Unlike SETD3 or METTL18, which methylates a unique substrate, METTL9 specifically recognizes an xHxH motif (H is for histidine and x denotes small residues.) and catalyzes the methylation of the second histidine. xHxH, as a known metal binding motif, is found in a wide range of metal binding proteins, suggesting the potential role of METTL9-dependent histidine methylation in mediating the metal binding capacities for those proteins. Based on the predicted METTL9 structure from AlphaFold11, we chose to mutate its surface-exposed hydrophobic residues to stabilize the protein. One METTL9 fragment (METTL946–318) with six mutations, named METTL9M6 afterwards, exhibited high solubility and homogeneity. In all METTL9M6 complexes, H1 and H-2 are snugly positioned into histidine-specific pockets, while x-1 forms hydrogen bond or hydrophobic interactions with METTL9M6 and x-3 stacks with the aromatic ring of METTL9M6 Tyr306.

Next, we solved the 2.10 Å structure of METTL9M6 bound with SAH and methylated SLC39A5 peptide, in which the peptide is well resolved with His375 methylated at the N1 atom, demonstrating the histidine N1-specific methylation activity of METTL9M6. The distance between the methyl group of His375me and SAH is 3.0 Å, indicating that it is a postreactive structure. The product-bound structure is identical to that of the substrate-bound structure, indicating that no remarkable conformational changes occur during catalysis. This finding is in contrast with our previously solved SETD3 structures, in which the imidazole ring of actin histidine rotates ~90° during catalysis. In contrast, H375A abolished the substrate binding affinity of METTL9, and the side chain of the substrate histidine did not change orientation during METTL9-mediated methyl transfer, suggesting their different substrate properties.

>[2x]HMAAGGRKENHQWYVCNREKLCESLQAVFVQSYLDQGTQIFLNNSIEKSGWAAIQAYHSAVSSAFSLAMSRTSINGLLGRGSMFVFSPDQFQRLLKINPDWKTHRLLDLGAGDGEVTKIMSPHFEEIYATELSETMIWQLQKKKYRVLGINEWQNTGFQYDVISCLNLLDRCDQPLTLLKDIRSVLEPTRGRVILALVLPFHPYVENVGGKWEKPSEILEIKGQNWEEQVNSLPEVFRKAGFVIEAFTRLPYLCEGDMYNDYYVLDDAVFVLKPV;>[2x]GHQGHSHGHQGGY>MSDKDSKNTPQVPEKLGLSRRGFLGASAVTGAAVAATALGGAVMTRESWAQAVKESKQKIHVGPGELDDYYGFWSGGHQGEVRVLGVPSMRELMRIPVFNVDSATGWGLTNESRHIMGDSAKFLNGDCHHPHISMTDGKYDGKYLFINDKANSRVARIRLDIMKCDKMITVPNVQAIHGLRLQKVPHTKYVFANAEFIIPHPNDGKVFDLQDENSYTMYNAIDAETMEMAFQVIVDGNLDNTDADYTGRFAAATCYNSEKAFDLGGMMRNERDWVVVFDIHAVEAAVKAGDFITLGDSKTPVLDGRKKDGKDSKFTRYVPVPKNPHGCNTSSDGKYFIAAGKLSPTCSMIAIDKLPDLFAGKLADPRDVIVGEPELGLGPLHTTFDGRGNAYTTLFIDSQVVKWNMEEAVRAYKGEKVNYIKQKLDVHYQPGHLHASLCETNEADGKWLVALSKFSKDRFLPVGPLHPENDQLIDISGDEMKLVHDGPTFAEPHDCIMARRDQIKTKKIWDRNDPFFAPTVEMAKKDGINLDTDNKVIRDGNKVRVYMTSMAPAFGVQEFTVKQGDEVTVTITNIDQIEDVSWGFVVVNHGVSMEISPQQTSSITFVADKPGLHWYYCSWFCHALHMEMVGRMMVEPAWSH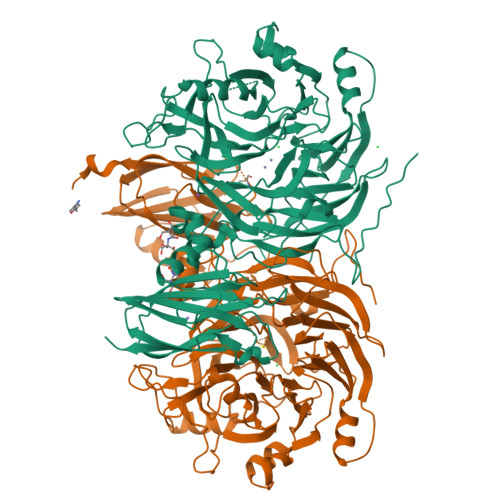PQFEK[2x]>[2x]MSKPQPIAAANWKCNGSQQSLSELID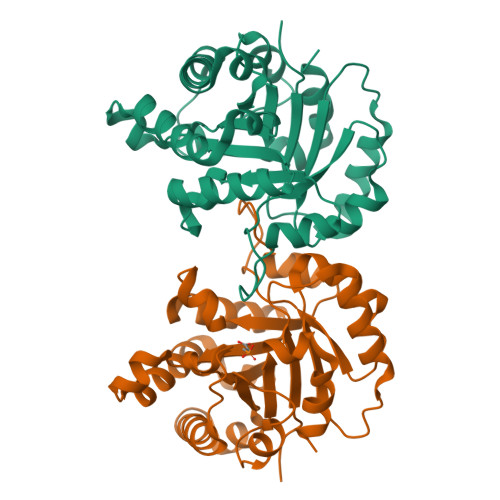LFNSTSINHDVQCVVASTFVHLAMTKERLSHPKFVIAAQNAIAKSGAFTGEVSLPILKDFGVNWIVLGHSERRAYYGETNEIVADKVAAAVASGFMVIACIGETLQERESGRTAVVVLTQIAAIAKKLKKADWAKVVIAYEPVWAIGTGKVATPQQAQEAHALIRSWVSSKIGADVAGELRILYGGSVNGKNARTLYQQRDVNGFLVGGASLKPEFVDIIKATQ(3S,6S)-3-ethyl-6-[(1H-indol-3-yl)methyl]piperazine-2,5-dione | C15 H17 N3 O2 | 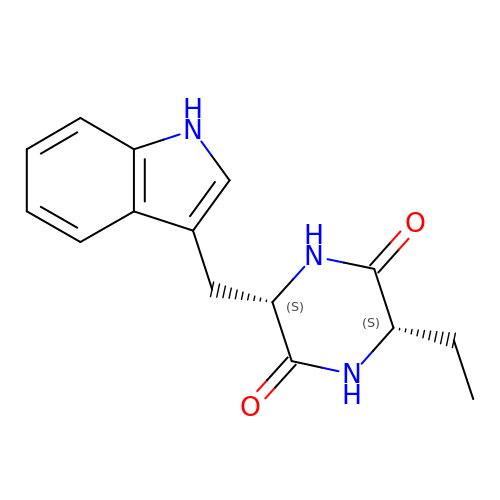BLROIZPIUOLTDB-AAEUAGOBSA-N The mitochondrial calcium uniporter is a highly selective multi-subunit Ca2+ channel of the inner mitochondrial membrane that serves as the major conduit for uptake of Ca2+ by mitochondria and controls ATP production in response to cytosolic Ca2+ signals. The protein MCU constitutes the pore of the uniporter through which Ca2+ ions flow and EMRE, a small transmembrane protein that associates with MCU, is necessary for Ca2+ uptake in metazoan organisms. Ca2+-dependent control is conferred by proteins that are unique to the uniporter − heterodimers of MICU1-MICU2 in most cells and of MICU1-MICU3 in neurons. At the ~100 nM resting level of [Ca2+]cytosol, MICU1-MICU2 and MICU1-MICU3 heterodimers prevent ion conduction through the channel, and they permit it when Ca2+ levels rise.

From biochemical analysis of the purified protein, and in acoord with a previous report that MICU1-MICU2 has an affinity for cardiolipin, we found that the heterodimer associates with lipid membranes and lipid nanodiscs that contain cardiolipin. This association is independent of Ca2+ - both Ca2+-free and Ca2+-bound heterodimers bind to liposomes. To investigate the conformational change in MICU1-MICU2 upon Ca2+ binding, we determined a cryo-EM structure of Ca2+-bound MICU1-MICU2 in complex with a lipid nanodisc containing cardiolipin at 3.1 Å resolution. The side of the heterodimer that associates with the nanodisc is the same as the one that faces the channel. The structure reveals a substantial conformational change upon Ca2+ binding that makes the heterodimer more compact and markedly more bent between MICU1 and MICU2. Ca2+ dependent rearrangements of the EF-hand motifs that involve their helix turn helix elements produce this bend. Ca2+ binding also induces a rotation of the UID relative to MICU1. Superimposing the Ca2+-bound MICU1-MICU2 structure on the UID in the resting holocomplex reveals that the Ca2+-induced conformational changes in the heterodimer would place hydrophilic regions of MICU2 within the membrane, which would be highly unfavorable thermodynamically (middle). Rather than inserting into the membrane, we hypothesize that the bending motion of MICU1-MICU2 acts like a lever against the membrane to pry MICU1 from the mouth of the pore when [Ca2+]IMS is elevated. The conformational changes would dislodge the UID from the blocking conformation, which would allow Ca2+ ions to permeate though the channel while [Ca2+]IMS remains elevated.

> GPTAAALEPHPEEKKKKRSGFRDRKVMEYENRIRAYSTPDKIFRYFATLKVISEPGEAEVFMTPEDFVRSITPNEKQPEHLGLDQYIIKRFDGKKISQEREKFADEGSIFYTLGECGLISFSDYIFLTTVLSTPQRNFEIAFKMFDLNGDGEVDMEEFEQVQSIIRSQTSMGMRHRDRPTTGNTLKSGLCSALTTYFFGADLKGKLTIKNFLEFQRKLQHDVLKLEFERHDPVDGRITERQFGGMLLAYSGVQSKKLTAMQRQLKKHFKEGKGLTFQEVENFFTFLKNINDVDTALSFYHMAGASLDKVTMQQVARTVAKVELSDHVCDVVFALFDCDGNGELSNKEFVSIMKQRLMRGLEKPKDMGFTRLMQAMWKCAQETAWDFALPKQSNW;> HHSRVSVAARDGSFTVSAQKNVEHGIIYIGKPSLRKQRFMQFSSLEHEGEYYMTPRDFLFSVMFEQMERKTSVKKLTKKDIEDTLSGIQTAGCGSTFFRDLGDKGLISYTEYLFLLTILTKPHSGFHVAFKMLDTDGNEMIEKREFFKLQKIISKQDDLMTVKTNETGYQEAIVKEPEINTTLQMRFFGKRGQRKLHYKEFRRFMENLQTEIQEMEFLQFSKGLSFMRKEDFAEWLLFFTNTENKDIYWKNVREKLSAGESISLDEFKSFCHFTTHLEDFAIAMQMFSLAHRPVRLAEFKRAVKVATGQELSNNILDTVFKIFDLDGDECLSHEEFLGVLKNRMHRGLWVPQHQSIQEYWKCVKKESIKGVKEVWKQAGKGLF>MAEIP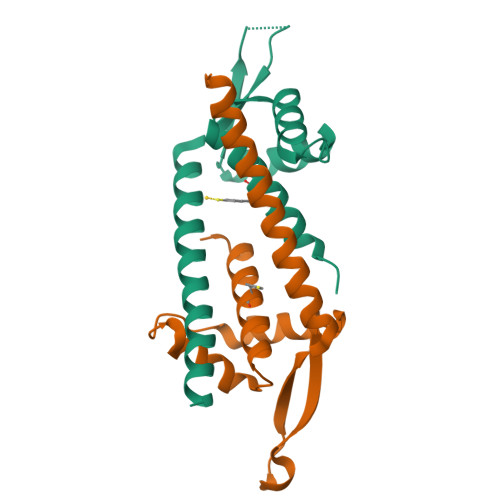KEMLRAQTNAILLNVLKQGDNYVYGIIKQVKEASNGEMELNEATLYTIFKRLEKDGIISSYWGDESQGGRRKYYRLTEIGHENMRLAFESWSRVDKIIENLEANKKSEAIKSRWSHPQFEK[2x]>[4x]SMQRTVARDITLLECVGKGRYGEVWRGSWQGENVAVKIFSSRDEKSWFRETELYNTVMLRHENILGFIA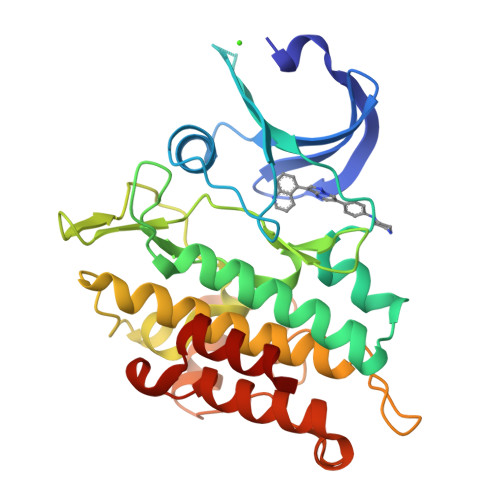SDMTSRHSSTQLWLITHYHEMGSLYDYLQLTTLDTVSCLRIVLSIASGLAHLHIEIFGTQGKPAIAHRDLKSKNILVKKNGQCCIADLGLAVMHSQSTNQLDVGNNPRVGTKRYMAPEVLDETIQVDCFDSYKRVDIWAFGLVLWEVARRMVSNGIVEDYKPPFYDVVPNDPSFEDMRKVVCVDQQRPNIPNRWFSDPTLTSLAKLMKECWYQNPSARLTALRIKKTLTKID> AANDNNVEWNGLFHDQGPLFDNAPEPTSTQSVTLKLRTFKGDITSANIKYWDTADNAFHWVPMVWDSNDPTGTFDYWKGTIPASPSIKYYRFQINDGTSTAWYNGNGPSSTEPNADDFYIIPNFKTPDWLKNGVMYQIFPDRFYNGDSSNDVQTGSYTYNGTPTEKKAWGSSVYADPGYDNSLVFFGGDLAGIDQKLGYIKKTLGANILYLNPIFKAPTNHKYDTQDYMAVDPAFGDNSTLQTLINDIHSTANGPKGYLILDGVFNHTGDSHPWFDKYNNFSSQGAYESQSSPWYNYYTFYTWPDSYASFLGFNSLPKLNYGNSGSAVRGVIYNNSNSVAKTYLNPPYSVDGWRLNAAQYVDANGNNGSDVTNHQIWSEFRNAVKGVNSNAAIIGQYWGNANPWTAQGNQWDAATNFDGFTQPVSEWITGKDYQNNSASISTTQFDSWLRGTRANYPTNVQQSMMNFLSNHDITRFATRSGGDLWKTYLALIFQMTYVGTPTIYYGDEYGMQGGADPDNRRSFDWSQATPSNSAVALTQKLITIRNQYPALRTGSFMTLITDDTNKIYSYGRFDNVNRIAVVLNNDSVSHTVNVPVWQLS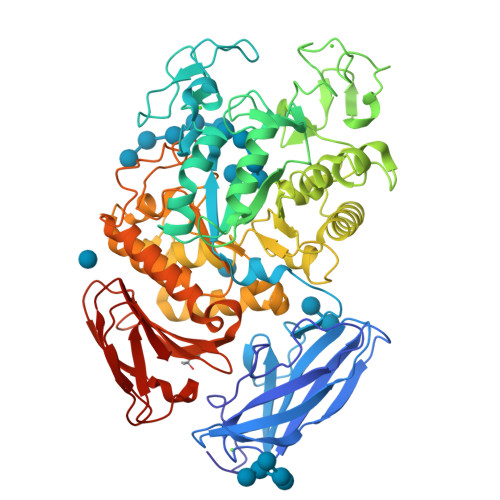MPNGSTVTDKITGHSYTVQNGMVTVAVDGHYGAVLAQ>MAFNGAQTVIQKISWLRTAIAFLKGYMETTGATKKELEQVEKLKERVDEIATAVNWDVYAQYARGDFNLLSDDEYKEIQKALLVLEDIKEQIIVEMLRVGLAQGQMGTLKISDYLDSLDSHHHHHH[2x]

Pyrococcus abyssi virus 1 (PAV1) was the first virus particle infecting a hyperthermophilic Euryarchaeota (Pyrococcus abyssi strain GE23) that has been isolated and characterized. The 18 kb dsDNA genome of PAV1 contains 25 predicted genes, most of them of unknown function. We present here the X-ray crystal structure of a putative ORFan protein PAV1-137, to our knowledge the first for a euryarchaeal viral protein. The fold of PAV1-137 is a four-α-helical bundle analogous to those found in some eukaryotic adhesion proteins such as focal adhesion kinase, suggesting that PAV1-137 is involved in protein-protein interactions.

We purified the C-terminal His-tagged protein from a genetic construct deleted for the 14 first residues because sequence analysis predicted an unstructured conformation for this N-terminal region. Two copies of PAV1-137 are present in the asymmetric unit and their structures are almost identical (root mean square deviation = 0.5 Å). PAV1-137 contains four amphipathic helices that are organized as a helical bundle. The three N-terminal helices form a parallel up and down configuration while the C-terminal helix is shorter and packs with an angle of about 45° against helices 1 and 3. The core of the 3 helices is very hydrophobic consisting mainly of branched aliphatic amino acids. The connection between helices 3 and 4 is a longer stretch, resulting in a less tight packing of helix 4 compared to the other helices. The A and B monomers in the asymmetrical unit form a two-fold symmetrical dimer and the symmetry axis runs perpendicular to the direction of the long helices. The dimer interface involves helices 1, 2, and 4. Dimerisation buries 1278 Å2 per monomer corresponding to 17% of the solvent accessible surface area. The interface is more hydrophilic than the core of the helical bundle and is stabilized by 9 hydrogen bonds, mainly between side chain and side or main chain atoms.6-(dimethylamino)-2-(2-{[(5-methyl-1,3,4-thiadiazol-2-yl)methyl]amino}ethyl)-1H-benzo[de]isoquinoline-1,3(2H)-dione | C20 H21 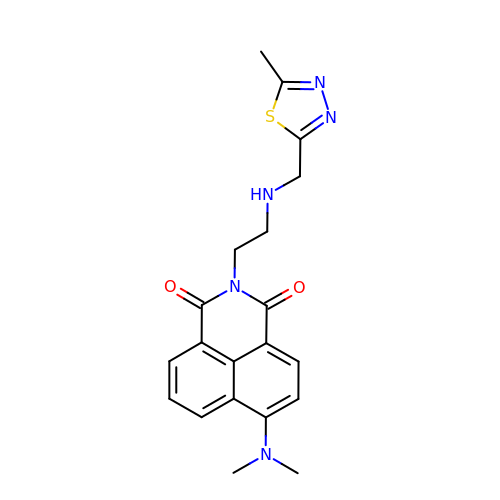N5 O2 S | MZVBLDCRQKXSHR-UHFFFAOYSA-N> HHHHHHENLYFQGMDIIFYHPTFDTQWWIEALRKAIPQARVRAWKSGDNDSADYALVFHPPVEMLAGRDLKAVFALGAGVDSILSKLQAHPEMLNPSVPL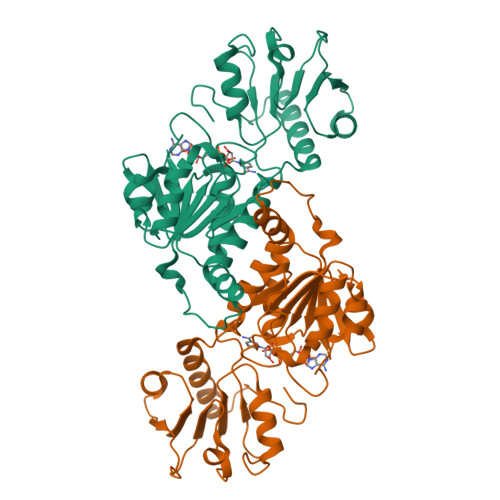FRLEDTGMGEQMQEYAVSQVLHWFRRFDDYRIQQNSSHWQPLPEYHREDFTIGILGAGVLGSKVAQSLQTWRFPLRCWSRTRKSWPGVQSFAGREELSAFLSQCRVLINLLPNTPETVGIINQQLLEKLPDGAYLLNLARGVHVVEDDLLAALDSGKVKGAMLDVFNREPLPPESPLWQHPRVTITPHVAAITRPAEAVEYISRTIAQLEKGEKVCGQVDRARGY PcyA, a ferredoxin-dependent bilin pigment reductase, catalyzes the site-specific reduction of the two vinyl groups of biliverdin (BV), producing phycocyanobilin. PcyA catalyzes a two-step reduction reaction: in the first step, the D-ring vinyl group of BV is reduced using two electrons and two protons to produce the reaction intermediate, 181, 182-dihydrobiliverdin (18EtBV), and in the second step, the A-ring of 18EtBV is reduced using two electrons and two protons to synthesize PCB. In the case of PcyA, three residues, namely, glutamate, histidine, and aspartate (Glu76, His88, and Asp105 in Synechocystis PcyA), present near the D- and A-rings of BV, are essential for the PcyA reaction. Here, we performed neutron crystallography and quantum chemical analysis of the D105N–BV and I86D–BV complexes to determine the protonation states of BV and the surrounding residues and study the correlation between the absorption spectra and protonation states around BV.

We recently found that Ile86, located near Glu76 and Asp105 in the three-dimensional (3D) structure, is important for the PcyA catalytic reaction. Although Ile86 is not a catalytic residue, its mutation to aspartic acid (I86D) disrupts the proton relay to BV. Thus, the reaction stops, and in I86D, similar to D105N, (an) electron(s) is/(are) donated to BV. During research to elucidate the reaction mechanism of PcyA, we also found that the I86D–BV complex exhibits a unique absorption spectrum with a sharp, high absorption peak around 730 nm. This peak is present as a shoulder peak in the WT PcyA–BV complex (hereafter referred to as the “WT–BV complex”), disappearing in the D105N–BV complex. Neutron structures elucidated that BV in the D105N mutant is in a neutral state, whereas that in the I86D mutant is dominantly in a protonated state. Glu76 and His88 showed different hydrogen bonding with surrounding residues compared with WT PcyA, further explaining why D105N and I86D have much lower activities for phycocyanobilin synthesis than the WT PcyA. The neutron structures of PcyA D105N–BV and I86D–BV at room temperature were refined to 2.10 Å and 2.00 Å resolutions, respectively. The R-factor and free R-factor for the D105N–BV structures were 16.51% and 18.00%, respectively, while those for the I86D–BV structures were 17.25% and 20.82%, respectively.

> MAVTDLSLTNSSLMPTLNPMIQQLALAIAASWQSLPLKPYQLPEDLGYVEGRLEGEKLVIENRCYQTPQFRKMHLELAKVGKGLDDLHCVMFPEPLYGLPLFGCDIVAGPGGVSAAIADLSPTQSDRQLPAAYQKSLAELGQPEFEQQRELPPWGEIFSEYCLFIRPSNVTEEERFVQRVVDFLQIHCHQSIVAEPLSEAQTLEHRQGQIHYCQQQQKNDKTRRVLEKAFGEAWAERYMSQVLFDVIQ> MDSKGSSQKGSRLLLLLVVSNLLLCQGVVSGSLQPLPPTAFTPNGTYLQHLARDPTSGTLYLG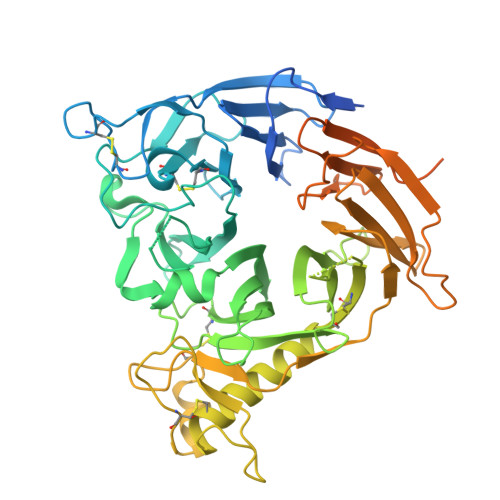ATNFLFQLSPGLQLEATVSTGPVLDSRDCLPPVMPDECPQAQPTNNPNQLLLVSPGALVVCGSVHQGVCEQRRLGQLEQLLLRPERPGDTQYVAANDPAVSTVGLVAQGLAGEPLLFVGRGYTSRGVGGGIPPITTRALWPPDPQAAFSYEETAKLAVGRLSEYSHHFVSAFARGASAYFLFLRRDLQAQSRAFRAYVSRVCLRDQHYYSYVELPLACEGGRYGLIQAAAVATSREVAHGEVLFAAFSSAAPPTVGRPPSAAAGASGASALCAFPLDEVDRLANRTRDACYTREGRAEDGTEVAYIEYDVNSDCAQLPVDTLDAYPCGSDHTPSPMASRVPLEATPILEWPGIQLTAVAVTMEDGHTIAFLGDSQGQLHRVYLGPGSDGHPYSTQSIQQGSAVSRDLTFDGTFEHLYVMTQSTLLKVPVASCAQHLDCASCLAHRDPYCGWCVLLGRCSRRSECSRGQGPEQWLWSFQPELGCLQTRENLYFQGKDGGGGGSHMGVAMPGAEDDVV>GHMDLKTAVFNAARDGKLRLLTKLLASKSKEEVSSLISEKTNGATPLLMAARYGHLDMVEFLLEQCSASIEVGGSVNFDGETIEGAPPLWAASAAGHLKVVQSLLNHGASVNNTTLTNSTPLRAACFDGHLEIVKYLVEHKADLEVSNRHGHTCLMISCYKGHKEIAQYLLEKGADVNRKSVKGNTALHDCAESGSLDIMKMLLMYCAKMEKDGYGMTPLLSASVTGHTNIVDFLTHHAQTSKTERINALELLGATFVDKKRDLLGALKYWKKAMNMRYSDRTNIISKPVPQTLIMAYDYAKEVNSAEELEGLIADPDEMRMQALLIRERILGPSHPDTS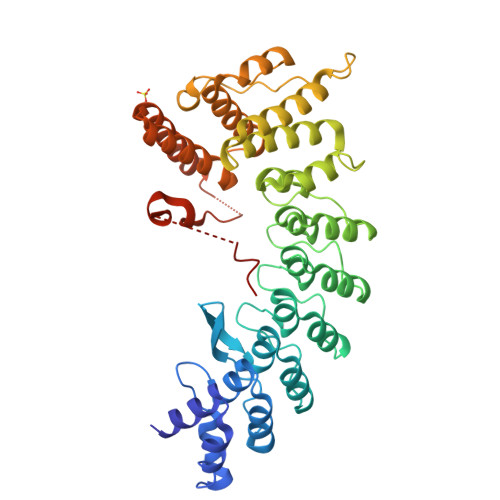YYIRYRGAVYADSGNFKRCINLWKYALDMQQSNLDPLSPMTASSLLSFAELFGGGSGGGSGGGSGGGSLNLPTQGRAR[2x]5-AMINO-NAPHTALENE-2-MONOSULFONATE | C10 H9 N O3 S | 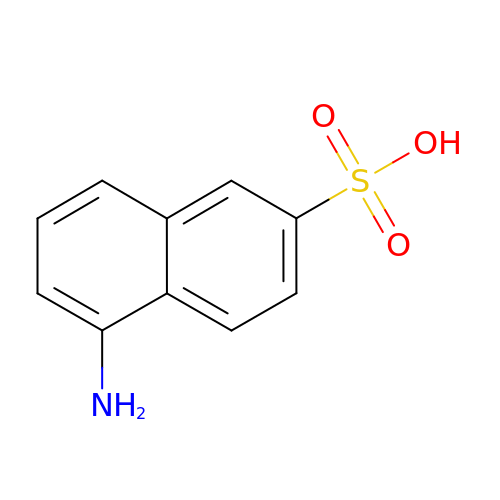UWPJYQYRSWYIGZ-UHFFFAOYSA-N> DFDCPSDWTAYDQHCYLAIGEPQNWYEAERFCTEQAKDGHLVSIQSREEGNFVAQLVSGFMHRSEIYVWIGLRDRREEQQCNPEWNDGSKIIYVNWKEGESKMCQGLTKWTNFHDWNNINCEDLYPFVCKFSAV;> CPLGWSSFDQHCY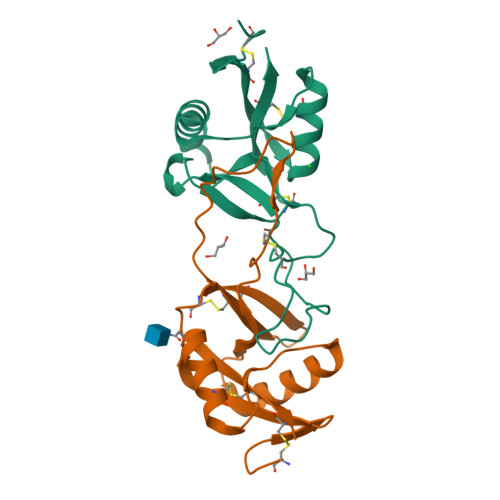KVFEPVKNWTEAEEICMQQHKGSRLASIHSSEEEAFVSKLASKALKFTSMWIGLNNPWKDCKWEWSDNARFDYKAWKRRPYCTVMVVKPDRIFWFTRGCEKSVSFVCKFLTDPAV>DDVIELTPSNFNREVIQSDSLWLVEFYAPWCGHCQRLTPEWKKAATALKDVVKVGAVDADKHHSLGGQYGVQGFPTIKIFGSNKNRPEDYQGGRTGEAIVDAALSALRQLVKDRLG[2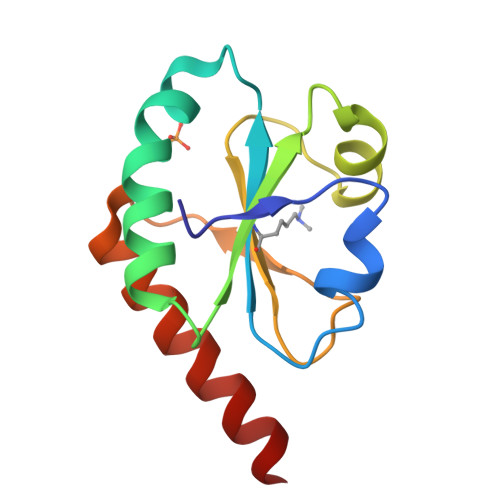x]>[8x]DDSRISSALQNLWTAAQAAMAAAVKAKAAEIAATKTPEEAKKVAEIAEKAIEIGKLAADAALGIAAAAGGKAVIAKMADGISPEKQAKYLAKFDAEAAAAKEGLAEAEKILKELLKEDPEAAKALTATALAAAAAAIAALLAAGLEHHHHHH

Pathogenic E. coli and Shigella spp. produce the outer membrane transporter ChuA, which binds host hemoglobin and extracts its heme cofactor, before importing heme into the cell. Heme extraction by ChuA is a dynamic process, with the transporter capable of rapidly extracting heme from hemoglobin in the absence of an external energy source, without forming a stable ChuA-hemoglobin complex. TBDTs consist of a 22-stranded transmembrane β-barrel with a pore occluded by a globular plug domain, which is transiently displaced during import. Using an AlphaFold2 model of ChuA as a target, we utilised RFdiffusion and ProteinMPNN to design binders targeting extracellular loops 7 and 8 of ChuA, which our model indicated were responsible for hemoglobin binding.

We expressed and purified four binders with the most prominent inhibition zones (A10, C8, G7 and H3). All binders inhibited αβHb and Mb-dependent growth of E. coliΔTBDT:ChuOP when spotted on agar, to a concentration of 250-500 nM for αβHb and 125-250 nM for Mb. To resolve how closely their computational design matches reality, we attempted to determine the crystal structures of A10, C8, G7 and H3 in isolation. Diffracting crystals were only obtained for binder C8, and the structure was solved at 2.46 Å. The crystal contained eight molecules per asymmetric unit, which have a pairwise similar RMSD of ~0.6 Å. This was comparable to the computational design of C8, which also had an RMSD of ~0.6 Å to the C8 molecules in the crystal structure, indicating that the predicted model closely matches the X-ray structure, once flexibility of the protein and experimental error are accounted for.1-[2,4-bis(chloranyl)-3-(trifluoromethyl)phenyl]-1,2,3-triazole | C9 H4 Cl2 F3 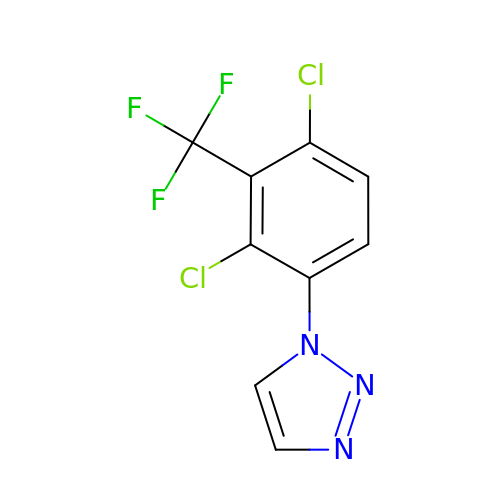N3 | XVFXHCLMGYJAQI-UHFFFAOYSA-N>MSVHVPGPHAMTIQELVDYVNARQKQGIYEEYEDIRRENPVGTFHCSMSPGNLEKNRYGDVPCLDQTRVKLTKRSGHTQTDYINASFMDGYKQKNAYIGTQGPLENTYRDFWLMVWEQKVLVIVMTTRFEEGGRRKCGQYWPLEKDSRIRFGFLTVTNLGVENMNHYKKTTLEIHNTEERQKRQVTHFQFLSWPDYGVPSSAASLIDFLRVVRNQQSLAVSNMGARSKGQCPEPPIVVHCSAGIGRTGTFCSLDICLAQLEELGTLNVFQTVSRMRTQRAFSIQTPEQYYFCYKAILEFAEKEGMVSAHHHHHH[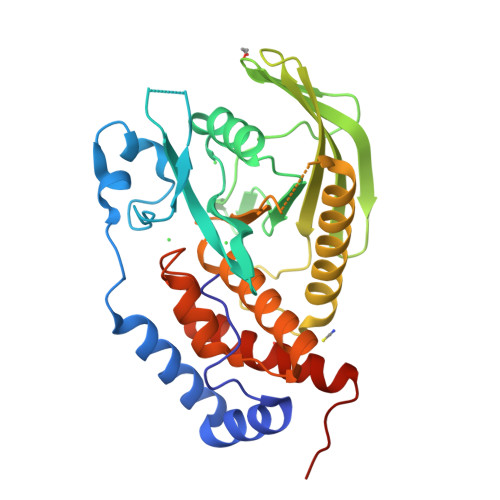2x]> MEEKVESTTTPDGPCVVSVQETEKWMEEAMRMAKEALENIEVPVGCLMVYNNEVVGKGRNEVNQTKNATRHAEMVAIDQVLDWCHQHGQSPSTVFEHTVLYVTVEPCIMCAAALRLMKIPLVVYGCQNERFGGCGSVLNIASADLPNTGRPFQCIPGYRAEEAVELLKTFYKQENPNAPKSKVRKKDCQKS;> MEPTSGFAEQPGPVKAESEEQEPAQWQALPVLSEQQSGAVELILAYAAPVLDKRQTSRLLREVSAVYPLPAQPHLKRVRPSRSAGGAQSSDLLLCLAGPSAGPRSLAELLPRPAVDPRGLGTPFLVPVPARPPLTRSQFEEARAHWPTSFHEDKQVTSALAGQLFSTQERAAMQTHMERAVCAAQRAAAQGLRAVGAVVVDPASDRVLATGHDCSSVASPLLHAVMVCIDLVAQGQGEDSLPYVCTGYDLYVTREPCVMCAMALVHARIQRVFYGAPSPDGALGTLFRVHARPDLNHRFQVFRGILEDQCRQLDPDP

The eukaryotic wobble adenosine-to-inosine modification is catalysed by the ADAT (ADAT2/ADAT3) complex that modifies up to eight tRNAs, requiring a full tRNA for activity. Our structure and associated enzymatic and biophysical analyses reveal that while ADAT2 active site catalyses the deamination reaction, ADAT3 active site is inactivated by the replacement by a valine of the glutamate involved in proton shuttling during catalysis but also by the capping of its zinc-binding pocket and the loss of tRNA recognition determinants. Our results show that the ADAT3 N-terminal domain adopts a fold that shares similarity with the ferredoxin-like domains (FLD) of other tRNA-modifying enzymes, yet with an additional specific structural subdomain, containing V128, which forms a loose interface between ADAT3 N- and C-terminal domains. ADAT3 N-terminal domain is essential for tRNA binding and deamination by ADAT and can rotate with respect to the catalytic domain formed by ADAT2 and the ADAT3 C-terminal domain, without affecting the structure of this latter catalytic domain.

The ADAT2/ADAT3-Δloop mutant complex could easily be produced and purified using the same experimental procedure developed for the wild-type (WT) complex, including the ion exchange chromatography step to remove the bound nucleic acids, and further crystallized. Two crystal forms were obtained, diffracting up to 2.1 and 3.0 Å, respectively. Crystals of ADAT2/ADAT3 that diffracted up to 3.0 Å resolution were obtained using a crystallization condition containing 0.1 M HEPES pH 7.0, 7% PEG 8000 and 8% ethylene glycol. Structure determination was made by collecting MAD data on ADAT zinc ions on the crystal form diffracting to 3.0 Å resolution. The combined MAD and model phases were then used to build the ADAT3 N-terminal domain. Surprisingly, the ADAT3-N domain is positioned differently in both structures with respect to the catalytic domain. Specifically, while the very N-terminus of ADAT3 interacts similarly with ADAT3-C in both structures, we observe a rotation of the ADAT3-N domains by around 90° with respect to each other. This rotation is only due to the movement of residues 34–39, the rest of ADAT3-N superposing very well, and possibly of residues 152–160 that are not seen in the electron density. Inspection of the location of the positively charged surfaces of ADAT3-N with respect to the tRNA revealed that these surfaces are completely opposite to the tRNA in the low resolution ADAT structure.>[3x]SRNTPDRRQRAAGDAERTQSMRLQQKINDLKPYVRHARGPIKAYGQAALDRASGAATSVSFAELDATHLDAMVYIENQRNPGLNLKHFRDHYYLIQALQSDGPSAFRAIF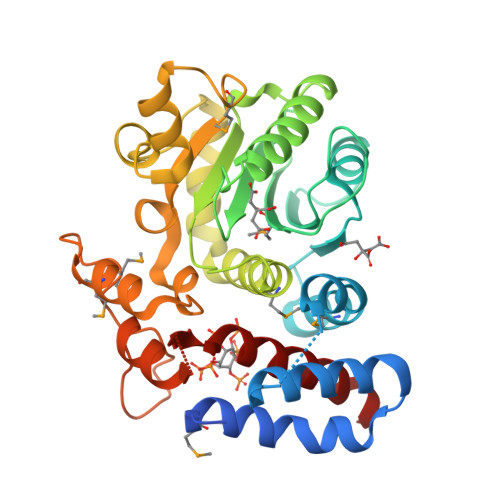PQTCPETGQTLKHHVMADVRLHQGGAPTIIITEPAVIVGARYQQLQRHNLTLEDLSESGVPLSQVAIIETQAAATSDDCVMYSLNYAIKAHKNAAQFDDIHHGLQHGTLSTESESRARTTLGALEASSSYSVMHEGAHAAFGADVLPVDFYKHGASLTQAYYLMKRPDGRMAGRVNSEGHSEAENLVQRNQAFRVKRRELLDDETPSNTQFSASIDGFRLQEIKRVLAAAQR> GKPLHEQLWYHGAIPRAEVAELLVHSGDFL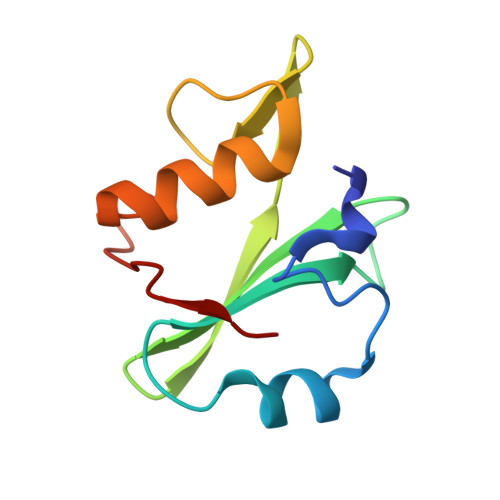VRESETVKGAYALSVLWDGLPRHFLIQSLDNLYRLEGEGFPSIPLLIDHLLSTQQPLTKKSGVVLHRAVP Fructose-1,6-bisphosphatase (FBPase) is a gluconeogenic enzyme that catalyzes the transformation of fructose 1,6-bisphosphate (F16BP) to fructose 6-phosphate (F6P) and phosphate. The gluconeogenic pathway of Leishmania converts metabolites into sugar phosphates to be used in the pentose phosphate pathway for synthesis of mannogen and glycoconjugates, which are essential for amastigote replication and virulence. Three crystal structures of LmFBPase have been determined: an apoenzyme structure that is in an unligated state, a structure bound with its catalytic product, and a structure in its allosterically inhibited form. The monomer core structure of LmFBPase has an α/β/α/β/α “club sandwich” topology, with two mixed β-sheets flanked by α-helices on both sides.

Manganese was demonstrated by TDA measurements to be a strong stabilizer of LmFBPase and was used as an additive to crystallize LmFBPase. Co-crystallization of LmFBPase with Mn2 + and the substrate F16BP resulted in crystals in which a catalytic product Pi and manganese atoms were found in each active site. The overall conformation is very similar to the apoenzyme structure, with an RMSD value of only 1.0 Å (based on Cα atoms). This structure also adopts a planar topology, which has no significant rotational movement of domains as analyzed by Dyndom. The dynamic loop (residues 52–71) was found to adopt an engaged conformation, in contrast to the apoenzyme structure where the dynamic loop was found to be disordered in two of the chains. The dynamic loop of LmFBPase was found to be stabilized in an engaged conformation in the presence of inorganic phosphate and manganese. The catalytic product Pi is found in the active site, surrounded by two (or possibly three) manganese atoms. Indeed, three electron density peaks were found in each active site of this LmFBPase/Mn/Pi structure; anomalous difference maps calculated from data collected at 1.89 Å (the absorption edge for Mn) showed clear peaks consistent with manganese ions at metal sites I and II. The electron density at site III is only slightly less than the electron density for the two manganese ions; however, there is no observable anomalous signal for site III, making potassium the more likely candidate. Similar coordination geometries around Mn-I and Mn-II are found in the LmFBPase crystal structures with Mn–O distances close to 2.2 Å.

>[4x]MDVRRTPTPTTLTQYIIKSQPPHSRGDFTLLMMAIQTSVKVIEKNIRRAGMKGMLGYIAGQSANATGDHQAKLDVISNIAFKAYLLSSTSVCVLGSEEEEQMIIAESGRRGDYLIFFDPLDGSSNIDANVSVGSIWGVWRLPKDTTINSVEDANAVIRMLKGTDMVSAGYAVYGSATNLVLTSGHGVDGFTLDPNIGEFILTHPHISIPKKRSIYSVNEGNYGKWEPWFKEYIDYLKMNKTTRYSARYIGSMVGDIHRTLLYGGIFCYPKDANQVEGKLRLLYEAAPMAMIVEQAGGKAVGSNGRILEQSITRLHQRTPVYFGSRQEVDLCMAFRDRNVKTEALAPTSSKL>MLTEEFVSAICGPPLSSNTAIAKDVGIYCHTLSPSYSVKSTFKKSSVPVNCLAVSDTHIFAGQHEKAYVHVYSRLRGNQEAFVALPERIRCLILIGDILVVGTTEGRLMLWEICTGRLVSTPARHVQAVSCVAATPSHVLTGSDDSDIHVWSLSQLLELDSAAEHEPLRTLANHRAAITALAVSPSDSADTNFCVSASKDKSCIIWNYQTGDALRTLIFPGYPLCMSLDPSSRAIFVSCEDSSLYVAEMFGEKPLLGPGSEDPSTVVQISTPFGATQPDVGPASCLSVSYDGTMLLTGHPRGQIMRWDISENKSPVELANLNAAVTNLIFVSPFLTSKPTKTVNIIKPSQAERAYTFTAQFEPMSFTKSRLDSLLNATGFPADALESAIVAFYQPVTQSAGDQELQRQNEELWEIINEQRALQKETLQRYVEAKSSR[2x];>MTAPPDLRVVCHRLASTPVDSLPRLCPLLINHVLRCGGPLSEPQDAKGKDRTSETAMLVHKFRTHITSLLTGKSPAGRFTAVCLIKAVIDVGGWESLRSAEPWIRGLIGVLQKPDPLSSKELSIVTLTKLYILLQDYQTLIREMATPTLPGYATACLQLIKPPASGRPLKVPLNFVDTVAWSLSKLVVLYSTTMRPFSGQIKSALRPYIAPTSSDNVVVPQSLKENSRNLLILLTYTAPKNGSSDEWVKAIRATILDCHTTADQVFRAVRESWESTTGYHIQPVNATGEPSGGGDSVDELPPWSGLQAGAERLTGLLEYLTAYFNNPTRAPVNVPLGELLDLTTRLTLVIPPSLGAEDSIETNPAIGRDEKAELWSALPDIHHAVLRLHCAIIRRLEANAIPLATDIIDQMVRVSTASKQLPSVRETAYILAKEILLLAGSTLPKLTVDILIPLIQSSCHDILTAAGHAQPAQSQSSVPVTASKQQKSSSPALTNADAFLPGQSSSSTPKTSTASPVSQAASALLPTFFTHLPQKHLPPDIRGLLDRTAILSHNQSAMLASCLHPYRDSRGRYYPSILPFLVRRFPRDESVEVLRSNLVKVGGSDASRGWDLSNGVTRDISYGREFAQEMISEEKGVVKEDETFAKEIEPVKSTAKPATSANAWGVEMELDVEHVNVAPIPETTNPFATVVGTTSQPSTLIQPACPSSPLKRKSDAEEFDEGSRPKRVDTGKAVSHPQMAVISSVPKPEEDKSDESSDSEGSVQIDMTLEDDEEDEEEEDE[2x]

The rixosome defined in Schizosaccharomyces pombe and humans performs diverse roles in pre‐ribosomal RNA processing and gene silencing. Here, we isolate and describe the conserved rixosome from Chaetomium thermophilum, which consists of two sub‐modules, the sphere‐like Rix1‐Ipi3‐Ipi1 and the butterfly‐like Las1‐Grc3 complex, connected by a flexible linker. The Rix1 complex of the rixosome utilizes Sda1 as landing platform on nucleoplasmic pre‐60S particles to wedge between the 5S rRNA tip and L1‐stalk, thereby facilitating the 180° rotation of the immature 5S RNP towards its mature conformation. Upon rixosome positioning, the other sub‐module with Las1 endonuclease and Grc3 polynucleotide‐kinase can reach a strategic position at the pre‐60S foot to cleave and 5′ phosphorylate the nearby ITS2 pre‐rRNA.

However, wild‐type ct PTF‐Las1 still co‐enriched Las1‐Grc3 together with Rix1‐Ipi1‐Ipi3, but not Rat1‐Rai1, and all five subunits remained stably associated during extended sucrose gradient centrifugation. Since the Rix1‐Ipi3‐Ipi1 complex is known to exhibit a large hollow sphere with a diameter of ~9 nm in yeast (Barrio‐Garcia et al, 2016; Kater et al, 2020) and the reconstituted ct Las1‐Grc3 heterodimer a butterfly‐like structure of 13 nm × 7 nm (Pillon et al, 2017), we conclude that we can observe the entire rixosome by electron microscopy. Once again, we observed the spherical density, which we attribute to the Rix1‐complex, and the butterfly‐shaped Las1‐Grc3, both arranged in such a way that the shorter edge of Las1‐Grc3 is preferentially oriented toward the Rix1 complex, with a distance of about 35 Å. While the cryo‐EM reconstruction of the complete rixosome could only be resolved at low resolution and did not reveal any apparent connecting density, both sub‐complexes could be resolved individually to resolutions of 2.9 Å (Rix1 complex) and 3.0 Å (Las1‐Grc3 complex). Accordingly, the Rix1 complex resembles essentially the structure observed on yeast pre‐60S particles, composed of two copies Rix1 and two copies Ipi3 (Kater et al, 2020), but without a rigidly bound Ipi1 subunit. This suggests a flexible connection of Ipi1 to the spherical Rix1‐Ipi3 core on the isolated rixosome, but on pre‐60S particles Ipi1 becomes fixed upon its binding to Sda1 (see below). The hollow sphere‐like structure is formed by two copies each of Rix1 and Ipi3. The Rix1 complex from C. thermophilum exhibits a highly similar structural organization when compared to the structures described in S. cerevisiae and human (Fig EV3; Pillon et al, 2019; Kater et al, 2020). Strikingly, AF2 multimer predicted with high consistency an interaction between the Las1‐CC and an intertwined bundle of two CC α‐helices formed by the two C‐termini of Ipi3 (Fig EV1B). The predictions agree with the previous finding that the Ipi3 CC domain is essential for Ipi3 homo‐dimerization (Barrio‐Garcia et al, 2016).>[8x]MSDWSGSVPANAENGKSTGLILKQGDT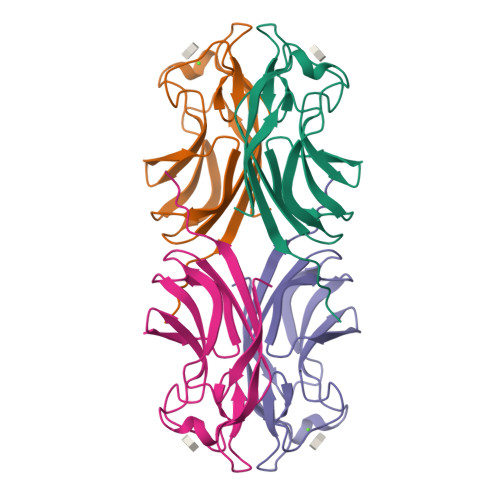ISVVAHGWVKYGRDNVEWAAPDGPVPNNPQPSSIATLVAKIANKKFAIGNGVLHKTVPVDGELILLFNDVPGTFGDNSGEFQVEVIIESRYSPLK>[5x]FRERLKELVVPKHVMDVVDEELSKLGLLDNHSSEFNVTRNYLDWLTSIPWGKYSNENLDLARAQAVLEEDHYGMEDVKKRILEFIAVSQLRGSTQGKILCFYGPPGVGKTSIARSIARALNREYFRFSVGGMTDVAEIKGHRRTYVGAMPGKIIQCLKKTKTENPLILIDEVDKIGRGYQGDPSSALLELLDPEQNANFLDHYLDVPVDLSKVLFICTANVTDTIPEPLRDRMEMINVSGYVAQEKLAIAERYLVPQARALCGLDESKAKLSSDVLTLLIKQYCRESGVRNLQKQVEKVLRKSAYKIVSGEAESVEVTPENLQDFVGKPVFTVERMYDVTPPGVVMGLAWTAMGGSTLFVETSLR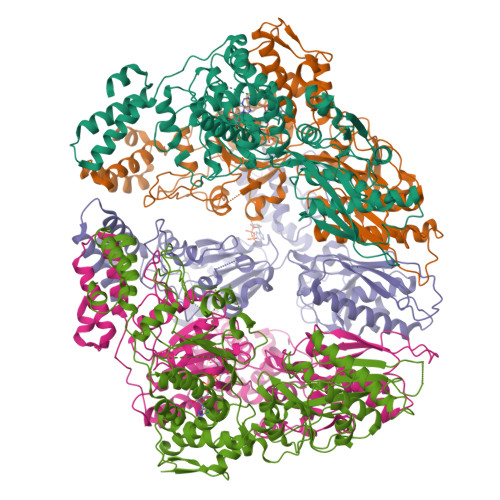RPQDKDAKGDKDGSLEVTGQLGEVMKESARIAYTFARAFLMQHAPANDYLVTSHIHLHVPEGATPKDGPSAGCTIVTALLSLAMGRPVRQNLAMTGEVSLTGKILPVGGIKEKTIAAKRAGVTCIVLPAENKKDFYDLAAFITEGLEVHFVEHYREIFDIAF9-[[4-[2,2-bis(fluoranyl)ethoxy]pyridin-2-yl]methyl]-2-chloranyl-purin-6-amine | C13 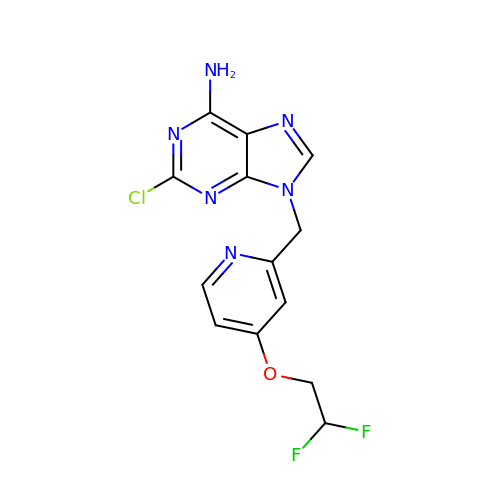H11 Cl F2 N6 O | SYPCZSDQCBMLSV-UHFFFAOYSA-N>MNSSLPSLRDVFANDFRIGAAVNPVTIEMQKQLLIDHVNSITAENHMKFEHLQPEEGKFTFQEADRIVDFACSHRMAVRGHTLVWHNQTPDWVFQDGQGHFVSRDVLLERMKCHISTVVRRYKGKIYCWDVINEAVADEGNELLRPSKWRQIIGDDFMEQAFLYAYEADPDALLFYNDYN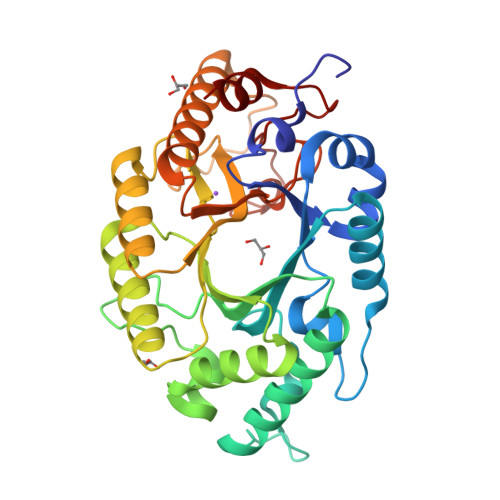ECFPEKREKIFALVKSLRDKGIPIHGIGMQAHWSLTRPSLDEIRAAIERYASLGVVLHITALDVSMFEFHDRRTDLAAPTSEMIERQAERYGQIFALFKEYRDVIQSVTFWGIADDHTWLDNFPVHGRKNWPLLFDEQHKPKPAFWRAVSV[2x]> GAGGGAGGGAGGGAAAAGGGG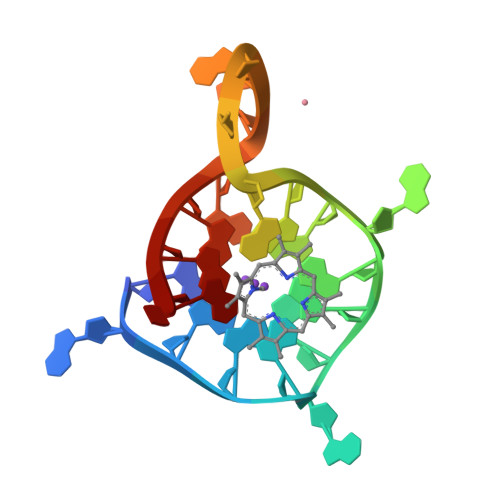A>AGAGADRTAATPAAANPAATEPVKWECPAGYEVKEGLNVDFPHKGMKRAFIVYPAKNVSGPAPVWVPMTGSVESTNDNLTVARSGANSILADHGYTVIAPVRACANQDPNIRGERCNGPGSNGWNWNPWFEGRAADPSGEHWKNDEGPDSSFFVAMVQCVGTKYKLDARRLFLGGISSGGTMTNRALLFRSNFWAGGLPIS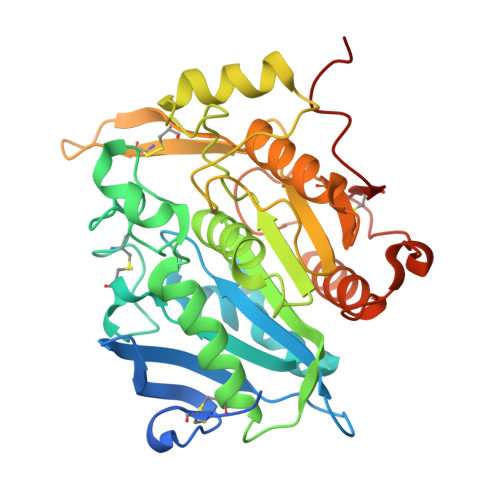GEWYVTSDDGTPLSFDDARAAVAAAPTKIHQGRVGPYPLPAKVGPLIVMTVWGGEKDLWNCTRPDGSRFLCADYRPSTQAGSNFFSAQPDVVHVACSSTHGHMWPQLNTQEFNRWALDTLASHPKGSDPRSFKLTQPPEGYTCHVGPFTGLYASAWSHPQFEK[2x]> M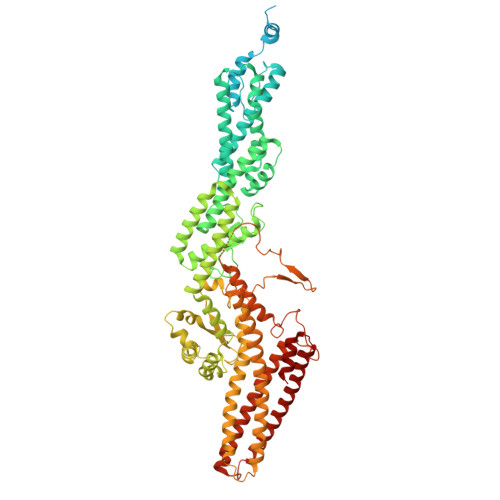ELEPTLFGIIEALAPQLLSQSHLQTFVSDVVNLLRSSTKSATQLGPLIDFYKLQSLDSPETTIMWHKIEKFLDALFGIQNTDDMVKYLSVFQSLLPSNYRAKIVQKSSGLNMENLANHEHLLSPVRAPSIYTEASFENMDRFSERRSMVSSPNRYVPSSTYSSVTLRQLSNPYYVNTIPEEDILKYVSYTLLATTSALFPFDHEQIQIPSKIPNFESGLLHLIFEAGLLYQSLGYKVEKFRMLNISPMKKALIIEISEELQNYTAFVNNLVSSGTVVSLKSLYREIYENIIRLRIYCRFTEHLEELSGDTFLIELNIFKSHGDLTIRKIATNLFNSMISLYYEYLMNWLTKGLLRATYGEFFIAENTDTNGTDDDFIYHIPIEFNQERVPAFIPKELAYKIFMIGKSYIFLEKYCKEVQWTNEFSKKYHVLYQSNSYRGISTNFFEIINDQYSEIVNHTNQILNQKFHYRDVVFALKNILLMGKSDFMDALIEKANDILATPSDSLPNYKLTRVLQEAVQLSSLRHLMNSPRNSSVINGLDARVLDLGHGSVGWDVFTLDYILYPPLSLVLNVNRPFGRKEYLRIFNFLWRFKKNNYFYQKEMLKSNDIIRSFKKIRGYNPLIRDIINKLSRISILRTQFQQFNSKMESYYLNCIIEENFKEMTRKLQRTENKSQNQFDLIRLNNGTIELNGILTPKAEVLTKSSSSKPQKHAIEKTLNIDELESVHNTFLTNILSHKLFATNTSEISVGDYSGQPYPTSLVLLLNSVYEFVKVYCNLNDIGYEIFIKMNLNDHEASNGLLGKFNTNLKEIVSQYKNFKDRLYIFRADLKNDGDEELFLLSKSLR> KQAFLILCLLSAAFAPICVGIVFLGFTPDHHCQSPGVAELSQRCGWSPAEELNYTVPGLGPAGEAFLGQCRRYEVDWNQSALSCVDPLASLATNRSHLPLGPCQDGWVYDTPGSSIVTEFNLVCADSWKLDLFQSCLNAGFLFGSLGVGYFADRFGRKLCLLGTVLVNAVSGVLMAFSPNYMSMLLFRLLQGLVSKGNWMAGYTLITEFVGSGSRRTVAIMYQMAFTVGLVALTGLAYALPHWRWLQLAVSLPTFLFLLYYWCVPESPRWLLSQKRNTEAIKIMDHIAQKNGKLPPADLKMLSLEEDVTEKLSPSFADLFRTPRLRKRTFILMYLWFTDSVLYQGLILHMGATSGNLYLDFLYSALVEIPGAFIALITIDRVGRIYPMAMSNLLAGAACLVMIFISPDLHWLNII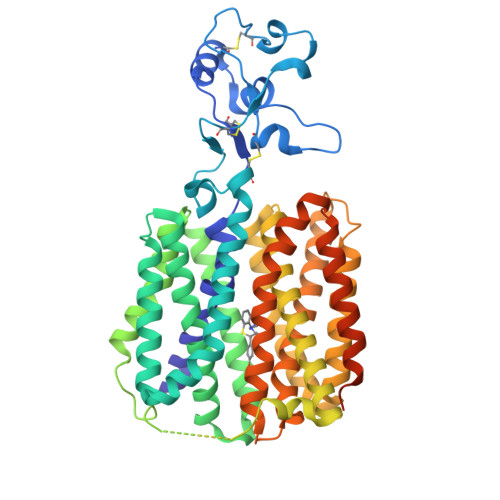IMCVGRMGITIAIQMICLVNAELYPTFVRNLGVMVCSSLCDIGGIITPFIVFRLREVWQALPLILFAVLGLLAAGVTLLLPETKGVALPETMKDAENLGRKAKPKENTIYLKVQTSEPSGT7-(3,5-DITERT-BUTYLPHENYL)-3-METHYLOCTA-2,4,6-TRIENOIC ACID | 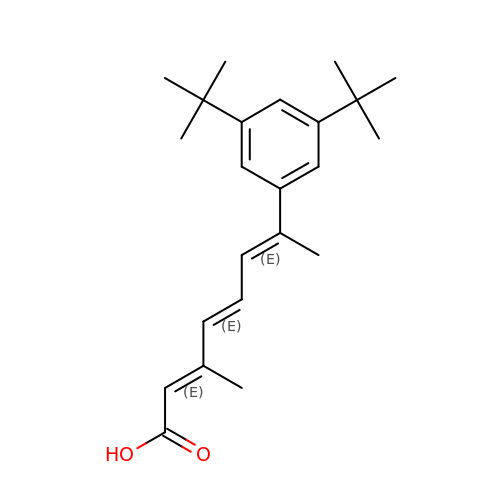C23 H32 O2 | JMPZTWDLOGTBPM-OUQSKUGOSA-N cyclopeptin | C17 H16 N2 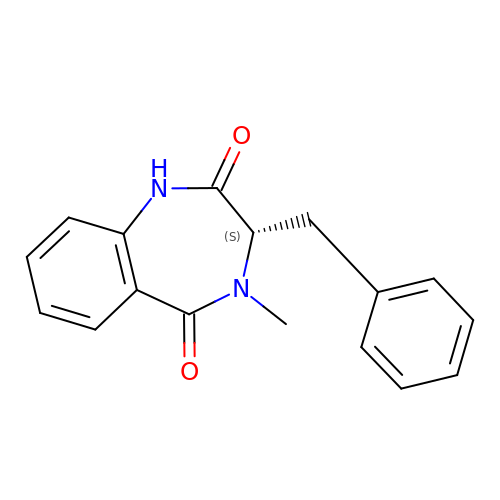O2 | KSQNKZMAMGACTL-HNNXBMFYSA-N> KTGLHFGRLSLRSLTAYAPNLMLWGGASMLGLFVFTE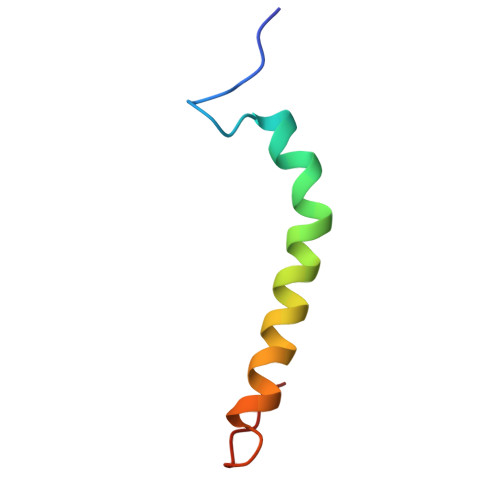GWPKFQD> GSHMASMSKDEVKREAKDTDGNPEIKGERRRLHSEIQSGSLANNIKKSTVI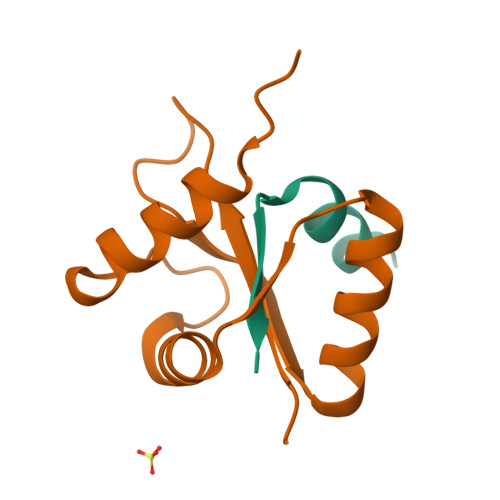VKN;> PTHIAICLYYKLGETPLPLVIETGKDAKALQIIKLAELYDIPVIEDIPLARSLDKNIHKGQYITEDFFEPVAQLIRIAIDLDY> MIPSITAYSKNGLKIE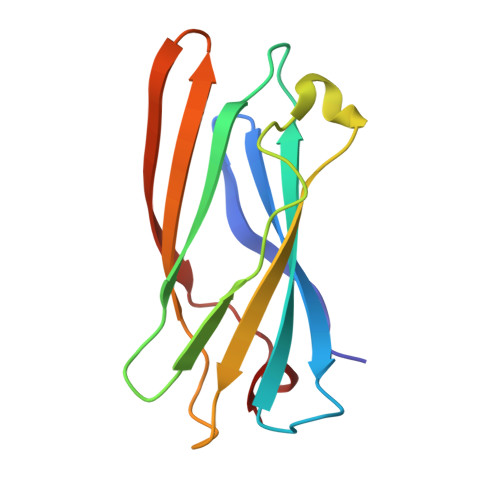FTFERSNTNPSVTVITIQASNSTELDMTDFVFQAAVPKTFQLQELSPSSSVVPAFNTGTITQVIKVLNPQKQQLRMRIKLTYNHKGSAMQDLAEVNNFPPQSWQ> AQSVPYGISQIKAPALHSQGYTGSNVKVAVIDSGIDSSHPDLNVRGGASFVPSETNPYQDGSSHGTHVAGTIAALNNSIGVLGVSPSASLYAVKVLDSTGSGQYSWIINGIEWAISNNMDVINMSLGGPTGSTALKTVVDKAVSSGIVVAAAAGNEGSSGSTSTVGYPAKYPSTIAVGAVNSSNQRASFSSAGSELDVMAPGVSIQSTLPGGTYGAYNGTCMATPHVAGAAALILSKHPTWTNAQVRDRLESTATYLGNSFYYGKGLINVQAAAQ;> EKKYIVGFKQTMSAMSSAKKKDVISQKGGKVEKQFKYVNAAAATLDEKAV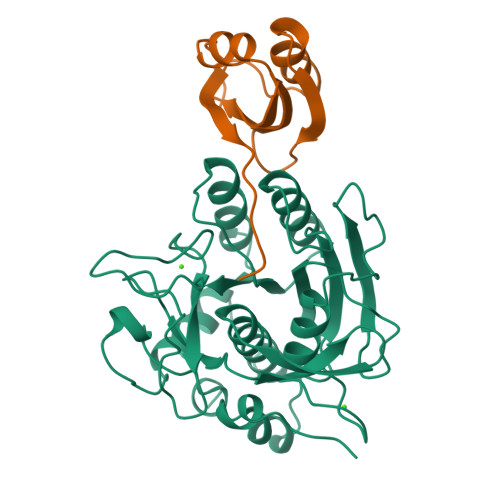KELKKDPSVAYVEEDHIAHEY>[2x]GHHHHHHHHHHSSGHIEGRHMKPSFSPRNYKALSEVQGWKQRMAAKELARQNMDLGFKLLKKLAFYNPGRNIFLSPLSISTAFSMLCLGAQDSTLDEIKQGFNFRKMPEKDLHEGFHYIIHELTQKTQDLKLSIGNTLFIDQRLQPQRKFLEDAKNFYSAETILTNFQNLEMAQKQINDFISQKTHGKINNLIENIDPGTVMLLANYIFFRARWKHEFDPNVTK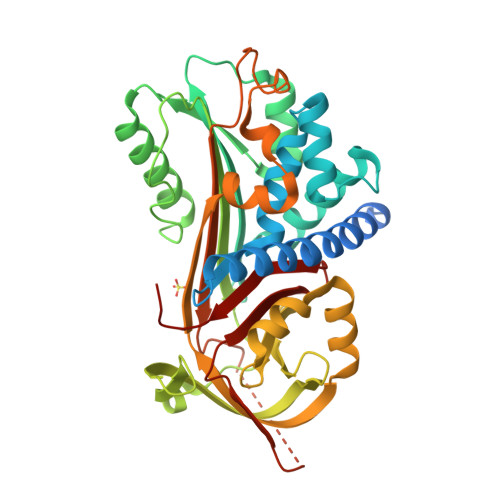EEDFFLEKNSSVKVPMMFRSGIYQVGYDDKLSCTILEIPYQKNITAIFILPDEGKLKHLEKGLQVDTFSRWKTLLSRRVVDVSVPRLHMTGTFDLKKTLSYIGVSKIFEEHGDLTKIAPHRSLKVGEAVHKAELKMDERGTEGAAGTGAQTLPMETPLVVKIDKPYLLLIYSEKIPSVLFLGKIVNPIGK> PSRKAKVKATLGEFDLRDYRNVEVLKRFLSET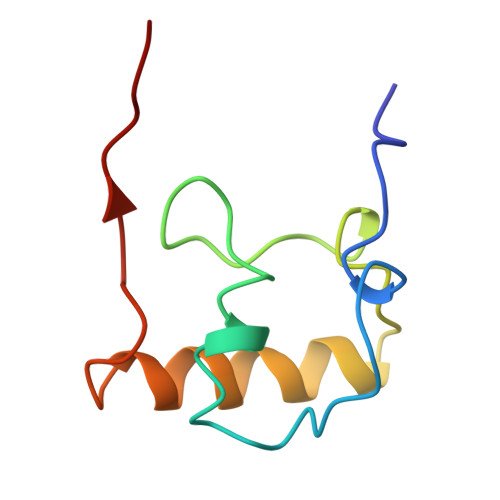GKILPRRRTGLSGKEQRILAKTIKRARILGLLPFTEKLVRK>SNAMGQITGAQIVARALKQQGVEYMFGIVGIPVIPIAMFAQREGIKFYGFRNEQSASYAAAAVGYLTGRPGVCLGVSGPGMIHGVAGMANAWSNCWPMILIGGANDSYQNGQGAFQEAPQIEAARPFAKYCARPDSLARLPFYVEQAVRTSIYGRPGAVYLDLPGDIITGAMEEEDVHFPPRCPDAPRMMAPQESIDAAMAALKSAERPLVIVGKGAAYSRAENEVREFLETTQLPYLASPMGKGVMPDDHPLSIAPARSAALLGADVILLMGARLNWMMHFGHPPRFDPKVRVIQMDISAEEIGTNVPTEVALVGDAKAITTQLNASLKQQPWQYPSETTWWTGLRKKIDENGATVAEMMADESVPMSYYRVYREIRDLIPNDAIIQNEGASTMDIGRTLMPNFLPRHRLDAGSFGTMGVGLGQAIAAAAVHPDKHVFCIEGDSAFGFSGMEVETAARYGMKNITFIIINNNGIGGGPDTLDPTRVPPSAYTPNAHYEKMAEIYGGKGYFVTEPSQLRPALEEAIKADKPAIVNIMISATSQRKPQQFAWLTR[8x]

One such enzyme is 2-hydroxyacyl-CoA lyase/synthase (HACL/S), which catalyzes the reversible cleavage of 2-hydroxyacyl-CoA (2hcCoA) into formyl-CoA (fCoA) and an aldehyde or ketone. Originally identified in the mammalian α-oxidation pathway of 3-methyl-branched fatty acids, HACL/S has demonstrated remarkable catalytic reversibility, as it is capable of condensing fCoA with various substrates covering a wide range of aldehydes and ketones with different carbon chain lengths. All the enzymes are tetramers, specifically dimers of dimers (α2), where α2 dimer represents a catalytical unit. The three domains have specific functions: the N-terminal domain binds the pyrimidine of ThDP (PYR), the middle domain has a regulatory function (R) and binds ADP, and the C-terminal domain binds the pyrophosphoryl group (PP) of ThDP.

We have determined ten high-resolution structures of enzymes from the HACL/S sub-family, including DhcHACL/S, CcHACL/S, TbHACL/S, CfhHACL/S, and ApbHACL/S and measure kinetic parameters for all purified enzymes. Based on the kinetic characterization ApbHACL/S, DhcHACL/S and TbHACL/S are the top three variants that showed the highest catalytic efficiency toward acetaldehyde. All structures contain well-defined bound ThDP and ADP. All our HACL/S structures contain bound ADP in the R domain, which assumes the Rossmann fold nucleotide binding unit.> MEIKDLKRLARYNPEKMAK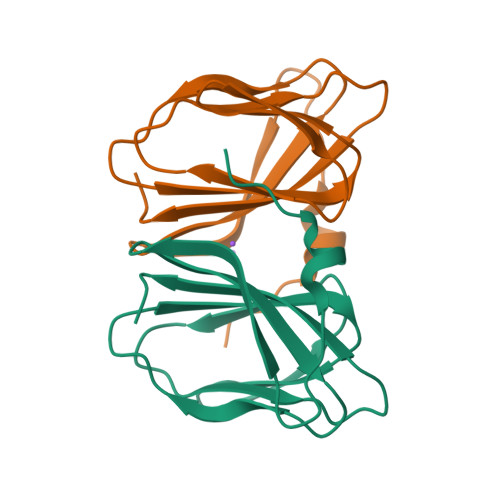IPVFQSERMLYDLYALLPGQAQKVHVHEGSDKVYYALEGEVVVRVGEEEALLAPGMAAFAPAGAPHGVRNESASPALLLVVTAPRP Human cytosolic prolyl-tRNA synthetase (HcProRS) catalyses the formation of the prolyl-tRNAPro, playing an important role in protein synthesis. Notably, glutamyl-prolyl-tRNA synthetase (EPRS) is a dual function enzyme that catalyses the formation of charged glutamyl-tRNA and prolyl-tRNA in the cytoplasm. The human ProRS (HcProRS) activity is located at the C-terminal region of this protein and inhibition of this enzyme has been recognized as a promising approach for treatment of HcProRS-related diseases. Inhibition of HcProRS activity has been shown to have potential benefits in the treatment of fibrosis, autoimmune diseases and cancer.

Pro binding induced the movement of the side chain of Arg1152 out of the ATP binding site, providing additional space to accommodate the binding of pyrazinamide derivatives.

>[2x]GAGEGQGPKKQTRLGLEAKKEENLADWYSQVITKSEMIEYHDISGCYILRPWAYAIWEAIKDFFDAEIKKLGVENCYFPMFVSQSALEKEKTHVADFAPEVAWVTRSGKTELAEPIAIRPTSETVMYPAYAKWVQSHRDLPIKLNQWCNVVRWEFKHPQPFLRTREFLWQEGHSAFATMEEAAEEVLQILDLYAQVYEELLAIPVVKGRKTEKEKFAGGDYTTTIEAFISASGRAIQGGTSHHLGQNFSKMFEIVFEDPKIPGEKQFAYQNSWGLTTRTIGVMTMVHGDNMGLVLPPRVACVQVVIIPCGITNALSEEDKEALIAKCNDYRRRLLSVNIRVRADLRDNYSPGWKFNHWELKGVPIRLEVGPRDMKSCQFVAVRRDTGEKLTVAENEAETKLQAILEDIQVTLFTRASEDLKTHMVVANTMEDFQKILDSGKIVQIPFCGEIDCEDWIKKTTARDQDLEPGAPSMGAKSLCIPFKPLCELQPGAKCVCGKNPAKYYTLFGRSY>[2x]ATTDAECLSKPAFDGTLSNVWKEGDSRYANFENCIYELSGIGIGYDNDTSWNGHWTPVRAADGSG;>[2x]DDIFGELSS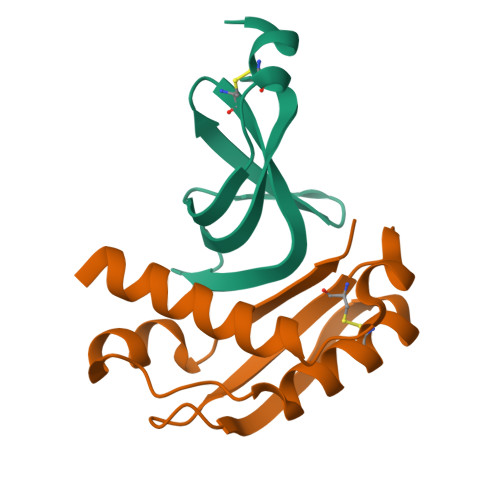GKNAPKTGGGAKGNNASPAGSGNTKNNGASGADINNYAGQIKSAIESKFYDASSYAGKTCTLRIKLAPDGMLLDIKPEGGDPALCQAALAAAKLAKIPKPPSQAVYEVFKNAPLDFKPAAAHHHHHH>[2x]MQNRQVANATKVAVAGASGYAGGEILRLLLGHPAYADGRLRIGALTAATSAGSTL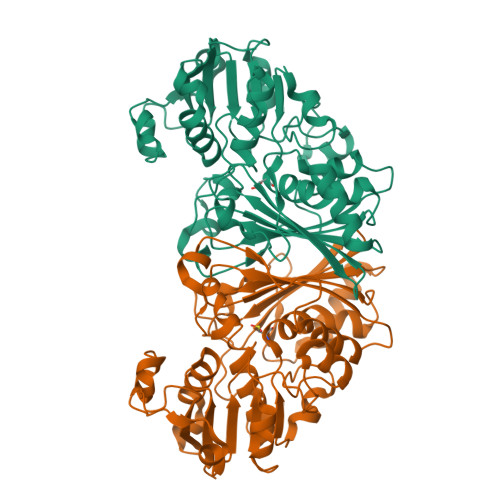GEHHPHLTPLAHRVVEPTEAAVLGGHDAVFLALPHGHSAVLAQQLSPETLIIDCGADFRLTDAAVWERFYGSSHAGSWPYGLPELPGARDQLRGTRRIAVPGCYPTAALLALFPALAADLIEPAVTVVAVSGTSGAGRAATTDLLGAEVIGSARAYNIAGVHRHTPEIAQGLRAVTDRDVSVSFTPVLIPASRGILATCTARTRSPLSQLRAAYEKAYHAEPFIYLMPEGQLPRTGAVIGSNAAHIAVAVDEDAQTFVAIAAIDNLVKGTAGAAVQSMNLALGWPETDGLSVVGVAP> SEFRRQTIRHSTREKDRGPTKATTTKLVYQIFDTFFAEQIEKDDREDKENAFKRRRCGVCEVCQQPECGKCKACKDMVKFGGSGRSKQACQERRCPNMAMKEADDDEEVDDNIPEMPSPKKMHQGKKKKQNKNRISWVGEAVKTDGKKSYYKKVCIDAETLEVGDCVSVIPDDSSKPLYLARVTALWEDSSNGQMFHAHWFCAGTDTVLGATSDPLELFLVDECEDMQLSYIHSKVKVIYKAPSENWA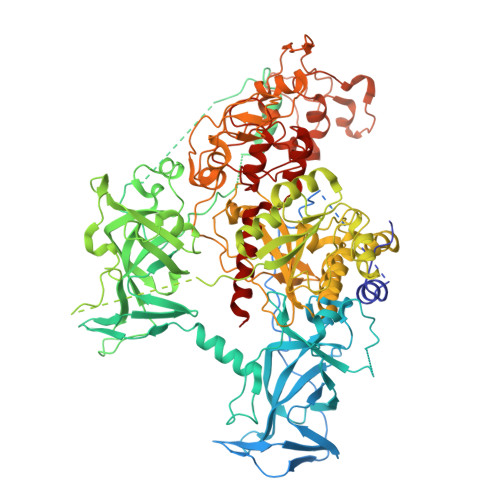MEGGMDPESLLEGDDGKTYFYQLWYDQDYARFESPPKTQPTEDNKFKFCVSCARLAEMRQKEIPRVLEQLEDLDSRVLYYSATKNGILYRVGDGVYLPPEAFTFNIKLSSPVKRPRKEPVDEDLYPEHYRKYSDYIKGSNLDAPEPYRIGRIKEIFCPKKSNGRPNETDIKIRVNKFYRPENTHKSTPASYHADINLLYWSDEEAVVDFKAVQGRCTVEYGEDLPECVQVYSMGGPNRFYFLEAYNAKSKSFEDPPNHARSPGNKGKGKGKGKGKPKSQACEPSEPEIEIKLPKLRTLDVFSGCGGLSEGFHQAGISDTLWAIEMWDPAAQAFRLNNPGSTVFTEDCNILLKLVMAGETTNSRGQRLPQKGDVEMLCGGPPCQGFSGMNRFNSRTYSKFKNSLVVSFLSYCDYYRPRFFLLENVRNFVSFKRSMVLKLTLRCLVRMGYQCTFGVLQAGQYGVAQTRRRAIILAAAPGEKLPLFPEPLHVFAPRACQLSVVVDDKKFVSNITRLSSGPFRTITVRDTMSDLPEVRNGASALEISYNGEPQSWFQRQLRGAQYQPILRDHICKDMSALVAARMRHIPLAPGSDWRDLPNIEVRLSDGTMARKLRYTHHDRKNGRSSSGALRGVCSCVEAGKACDPAARQFNTLIPWCLPHTGNRHNHWAGLYGRLEWDGFFSTTVTNPEPMGKQGRVLHPEQHRVVSVRECARSQGFPDTYRLFGNILDKHRQVGNAVPPPLAKAIGLEIKLCMLAKA> MLRWITAGESHGRALVAVVEGMVAGVHVTSADIADQLARRRLGYGRGARMTFERDAVTVLSGIRHGSTLGGPIAIEIGNTEWPKWETVMAADPVDPAELADVARNAPLTRPRPGHADYAGMLKYGFDDARPVLERASARETAARVAAGTVARAFLRQALGVEVLSHVISIGASAPYEGPPPRAEDLPAIDASPV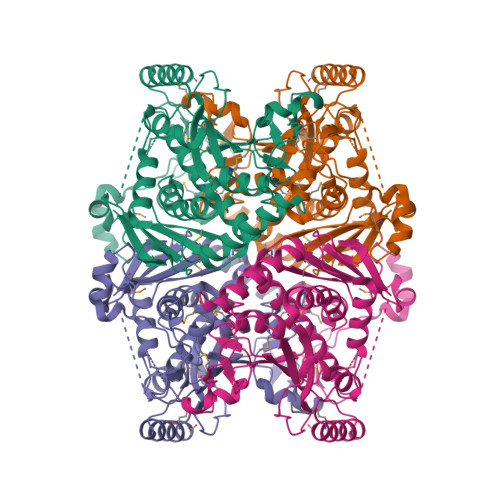RAYDKAAEADMIAQIEAAKKDGDTLGGVVEAVALGLPVGLGSFTSGDHRLDSQLAAAVMGIQAIKGVEIGDGFQTARRRGSRAHDEMYPGPDGVVRSTNRAGGLEGGMTNGQPLRVRAAMKPISTVPRALATVDLATGDEAVAIHQRSDVCAVPAAGVVVETMVALVLARAALEKFGGDSLAETQRNIAAYQRSVADREAPAARVSGHHHHHH>MNLESLLHWIYVAGMTIGALHFWSLSRNPRGVPQYEYLVAMFIPIWSGLAYMAMAIDQGKVEAAGQIAHYARYIDWMVTTPLLLLSLSWTAMQFIKKDWTLIGFLMSTQIVVITSGLIADLSERDWVRYLWYICGVCAFLIILWGIWNPLRAKTRTQSSELANLYDKLVTYFTVLWIGYPIVWIIGPSGFGWINQTIDTFLFCLLP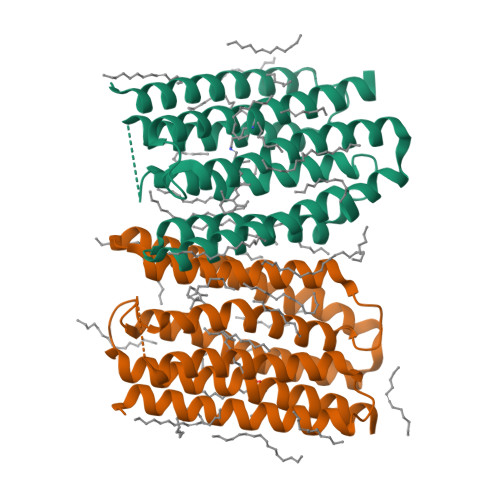FFSKVGFSFLELHGLRNLND[2x]>GPGYQMDIPKFKRLPRHIAIIPDGNRRWALARGLEKHEGYSSGIIPGLEVYDICVKIGIGEVTFFGFTQDNTKRPQIQRKAFTDACIKSVQEIAKRDAEILVVGNTNSDIFPEELLEYTKRTKVGKGKIKINFLINYGWYWDLTYAYDNSPDGKKMIENIASAEIPRVDLLIR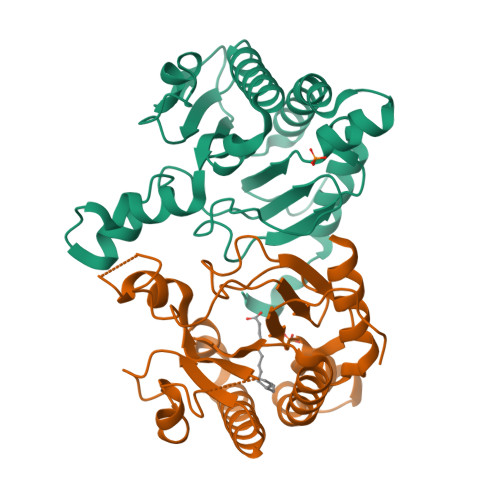WGGRCRLSGMLPVQTVYSDIYVVDEMWPDFKPEHLFKALEFYQNQDITLGG[2x]BbvCI, a Type IIT restriction endonuclease, recognizes and cleaves the seven base pair sequence 5′-CCTCAGC-3′, generating 3-base, 5′-overhangs. BbvCI is composed of two protein subunits, each containing one catalytic site. Either site can be inactivated by mutation resulting in enzyme variants that nick DNA in a strand-specific manner. Earlier mutagenesis of these residues confirmed their catalytic nature and demonstrated that the site in the R1 subunit cleaves the bottom strand of the target site, while the site in the R2 subunit cleaves the top strand.

However, after derivatization with heavy atom compounds ‘I3C’ or tantalum bromide, the space group was converted to C2221, with only two subunits (one dimer) in the asymmetric unit. We initially calculated MIR phases, built an initial structure, and conducted refinements using datasets corresponding to the latter (heavy-atom) space group, and then subsequently determined the final, higher resolution structure of the native (non-derivatized) protein in the original C222 space group via molecular replacement and phase extension. Initial attempts to model the density as a heterodimer of R1 and R2 subunits resulted in high values for the refinement R-factors, particularly RFree. In contrast, modeling the electron density as a homodimer comprising two copies of the R2 subunit resulted in satisfactory values for Rwork and Rfree (0.189/0.249, respectively), excellent correlation of the model to experimental electron density, and significantly improved geometric quality. Similar attempts to model and refine a homodimer of R1 subunits, instead, further degraded the model's performance and refinement statistics. Crystallization of the R2 subunit under such conditions revealed an elongated dimer with the two catalytic sites located on opposite sides. The first 115, and final 110, residues of each protein chain form a single protein domain of mixed alpha-beta topology built around the alpha-beta-alpha core common to PD-(D/E)XK REases. An intervening four-stranded, anti-parallel beta-sheet (residues 116–175) protrudes from this core. This interacts in a domain-swapped manner with its symmetry-mate in the opposing subunit, to form a dimer interface corresponding to an elongated beta-sheet. The molecule is saddle-shaped due to deep concave surfaces at the dimer interface, and there is no obvious region of contiguous positive surface charge that might accommodate a DNA duplex of seven or more base pairs.

>[2x]MFNQFNPLVYTHGGKLERKSKKDKTASKVFEEFGVMEAYNCWKEASLCIQQRDKDSVLKLVAALNTYKDAVEPIFDSRLNSAQEVLQPSILEEFFEYLFSRIDSIVGVNIPIRHPAKGYLSLSFNPHNIETLIQSPEYTVRAKDHDFIIGGSAKLTIQGHGGEGETTNIVVPAVAIECKRYLERNMLDECAGTAERLKRATPYCLYFVVAEYLKLDDGAPELTEIDEIYILRHQRNSERNKPGFKPNPIDGELIWDLYQEVMNHLGKIWWDPNSALQRGKVFNRP>[4x]GSVIDPSELTFVQEIGSGQFGLVHLGYWLNKDKVAIKTIREGAMSEEDFIEEAEVMMKLSHPKLVQLYGVCLEQAPICLVFEFMEHGCLSDYLRTQRGLFAAETLLG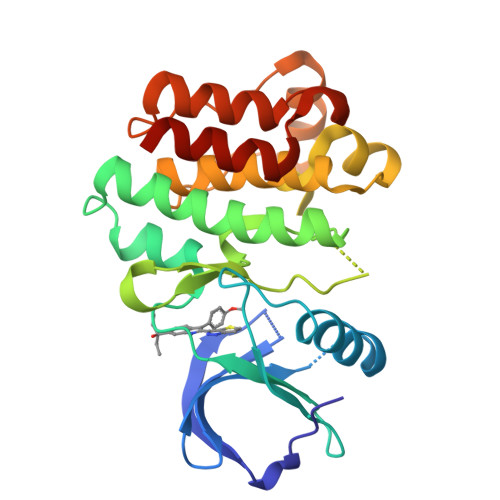MCLDVCEGMAYLEEACVIHRDLAARNCLVGENQVIKVSDFGMTRFVLDDQYTSSTGTKFPVKWASPEVFSFSRYSSKSDVWSFGVLMWEVFSEGKIPYENRSNSEVVEDISTGFRLYKPRLASTHVYQIMNHCWKERPEDRPAFSRLLRQLAEIAESGL>[2x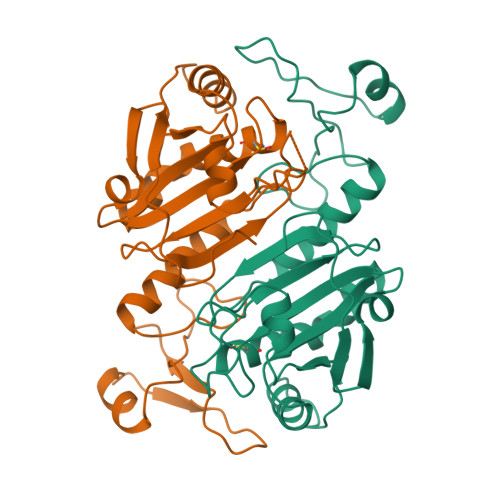]MPGGLLLGDVAPNFEANTTVGRIRFHDFLGDSWGILFSHPRDFTPVCTTELGRAAKLAPEFAKRNVKLIALSIDSVEDHLAWSKDINAYNSEEPTEKLPFPIIDDRNRELAILLGMLDPAEKDEKGMPVTARVVFVFGPDKKLKLSILYPATTGRNFDEILRVVISLQLTAEKRVATPVDWKDGDSVMVLPTIPEEEAKKLFPKGVFTKELPSGKKYLRYTPQP(3S)-4-{[4-(4-cyano-3-methylphenoxy)phenyl]acetyl}morpholine-3-carboxylic 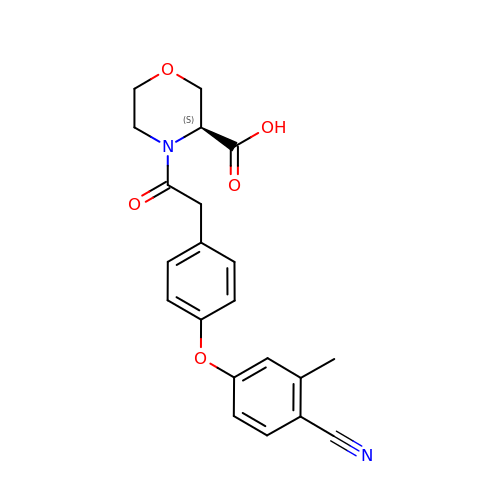acid | C21 H20 N2 O5 | AJUGJYIFDAVOIF-IBGZPJMESA-N> GSMTLSSNQYQLPLNVRPYTTTWCSQSPSCSNLLAIGHDTGITIYCASEEQTPGSTGLTLQELFTIQTGLPTLHLSFSSSCSYSENLHDGDGNVNSSPVYSLFLACVCQDNTVRLIITKNETIITQHVLGGKSGHHNFVNDIDIADVYSADNRLAEQVIASVGDDCTLIIWRLTDEGPILAGYPLSSPGISVQFRPSNPNQLIVGERNGNIRIFDWTLNLSAEENSQTELVKNPWLLTLNTLPLVNTCHSSGIASSLANVRWIGSDGSGILAMCKSGAWLRWNLFANNDYNEISDSTMKLGPKNLLPNVQGISLFPSLLGACPHPRYMDYFATAHSQHGLIQLINTYEKDSNSIPIQLGMPIVD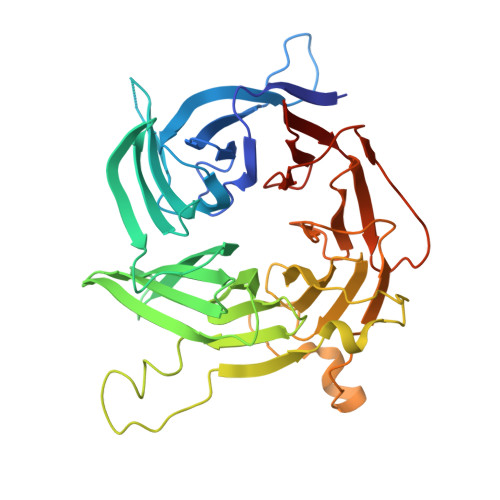FCWHQDGSHLAIATEGSVLLTRLMGFTRL>[2x]HMRVLVVPLPYPTHLMAMVPLCWALQASGHEVLIAAPPELQATAHGAGLTTAGIRGNDRTGDTGGTTQLRFPNPAFGQRDTEAGRQLWEQTASNVAQSSLDQLPEYLRLA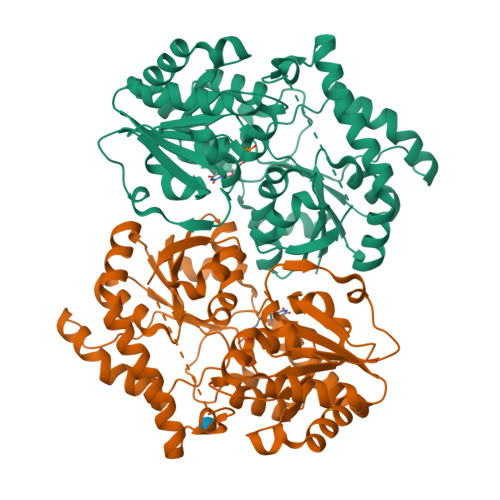EAWRPSVLLVDVCALIGRVLGGLLDLPVVLHRWGVDPTAGPFSDRAHELLDPVCRHHGLTGLPTPELILDPCPPSLQASDAPQGAPVQYVPYNGSGAFPAWGAARTSARRVCICMGRMVLNATGPAPLLRAVAAATELPGVEAVIAVPPEHRALLTDLPDNARIAESVPLNLFLRTCELVICAGGSGTAFTATRLGIPQLVLPQYFDQFDYARNLAAAGAGICLPDEQAQSDHEQFTDSIATVLGDTGFAAAAIKLSDEITAMPHPAALVRTLENTA>[2x]GKNMDTSAEPADVQANVSDSSRIEQEAIGMIEDFYEAYAASFMSTGKEALALGDSIKQKFLTKELIEKVDRLIEATDADPIIRAQDLGENDMKTLSVKHLNDNWYEVNYTSAKGSQYERAVS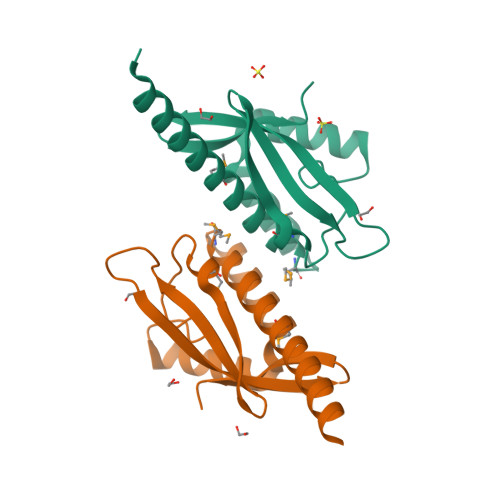IPVRVVNVDGQYLIDDITPEN D-gamma-glutamyl-L-cysteinyl-beta-alanine | C11 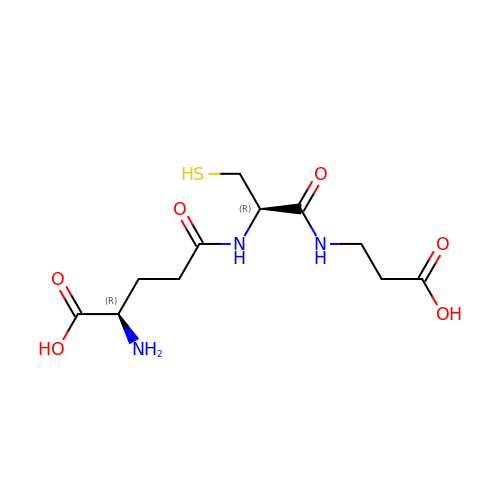H19 N3 O6 S | HKBNQXMLSMKLJV-RQJHMYQMSA-N> MAQKAPGVITCKAAVVWESSGPVVLEEIRVDPPKASEVRIKMLCASLCHTDVLCTKGFPIPLFPRIPGHEGVGVIESIGKDAKGLKPGDIVMPLYLGECGQCLNCKTGKTNLCHVYPPSFSGLMNDGTSRMSIARTGESIYHFASCSTWTEYAVADCNYVLKINPKISYPHASFLSCGFTTGFGATWRETQVSKGSSVAVFGIGTVGLGVIKGAQLQGASKIIGVDVNQYKAAKGKVFGMTDFINPKDHPDKSVSELVKELTHGLGVDHCFECTGVPSLLNEALEASKIGIGTVVPIGAGGEASVAINSLILFSGRTLKFTAFGGVRTQSDLPVIIDKCLNKEIQLDELLTHEIHLDNIQEAFEILKKPDCVKI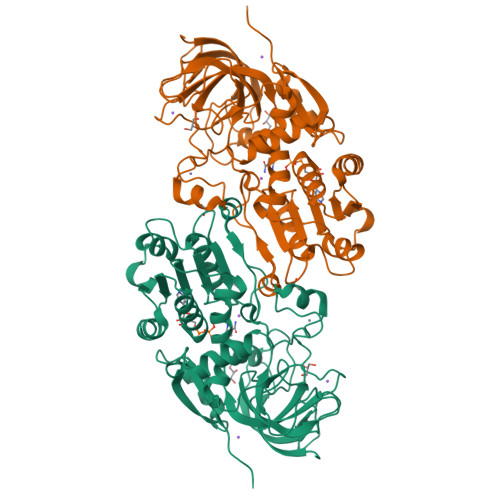LIKFLEHHHHHH>MRPLVIILMGSSSDMGHAEKIASELKTFGIEYAIRIGSAHKTAEHVVSMLKEYEALDRPKLYITIAGRSNALSGFVDGFVKGATIACPPPSDSFAGADIYSSLRMPSGISPALVLEPKNAALLAARIFSLYDKEIADSVKSY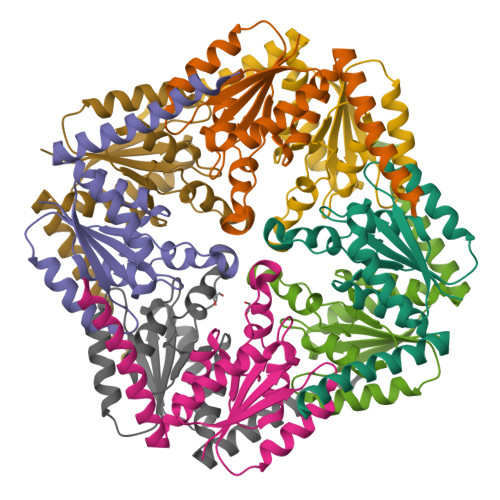MESNAQKIIEDDSKLKR[8x]5-phosphono-L-norvaline 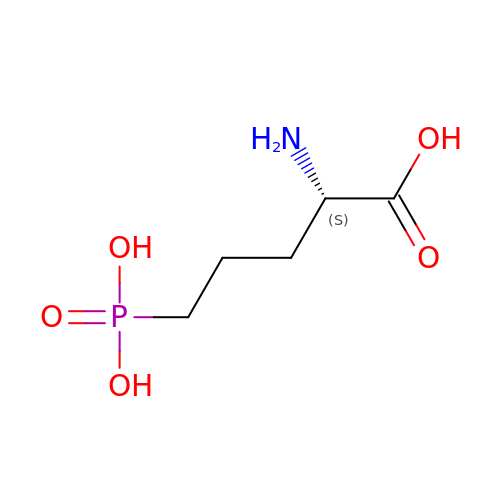| C5 H12 N O5 P | VOROEQBFPPIACJ-BYPYZUCNSA-N>[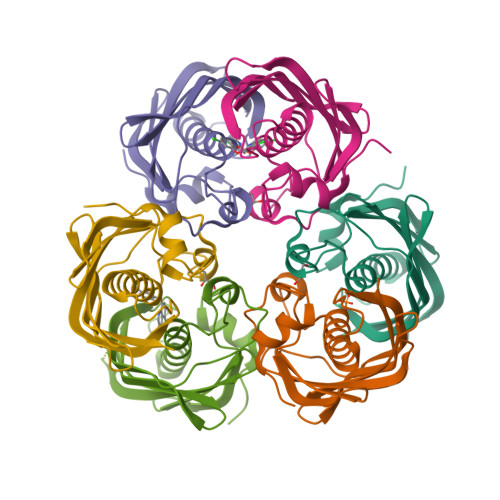24x]GSHMPNYDTSIDIEDIKKILPHRYPFLLVDKVIYMQPNKTIIGLKQVSTNEPFFNGHFPQKQIMPGVLQIEALAQLAGILCLKSDDSQKNNLFLFAGVDGVRWKKPVLPGDTLTMQANLISFKSSLGIAKLSGVGYVNGKVVINISEMTFALSK The Maintenance of Lipid Asymmetry (Mla) pathway is a multicomponent system found in all gram-negative bacteria that contributes to virulence, vesicle blebbing and preservation of the outer membrane barrier function. The pathway consists of an OM lipoprotein component (MlaA), found as part of a complex with either OmpC or OmpF7,8; a periplasmic GPL chaperone (MlaC) which shuttles GPL across the periplasm; and an IM ATP binding cassette (ABC) transporter complex (MlaFEDB). MlaFEDB consists of four proteins: MlaE an ABC permease protein; MlaD a membrane anchored MCE (mammalian cell entry) domain containing protein forming a homo-hexameric ring that faces the periplasm; MlaF, an ABC ATPase; and MlaB, a STAS (Sulfate Transporter and Anti-Sigma factor antagonist) domain protein proposed to have a regulatory function. Specifically, we report the structure of E. coli MlaC in complex with the MlaD hexamer, in two different stoichiometries (1:6 and 2:6, respectively), stabilised through the binding of cardiolipin.

Masked refinement and 3D classification, focusing on one MlaD hexamer, revealed two distinct species, one with a single MlaC bound to a MlaD32-183 hexamer, and another with two MlaC molecules bound, with final resolutions of 4.35 Å and 4.38 Å, respectively. In the MlaCD(2:6) structure, two MlaC molecules are bound on opposite sides of the MlaD32-183 hexamer, with overall 2-fold symmetry. Likewise, MlaCD(2:6) has a Cɑ RMSD of between 0.7 and 0.9 Å in the core fold across all pairwise protomer alignments, except for those positioned directly opposite in the hexamer, which have RMSDs as low as 0.3 Å in the core fold and 0.4 Å for the entire Cɑ trace. Further 2D and 3D classification of the data did not reveal any evidence for particles with additional copies of MlaC bound to the MlaD32-183 hexamer, or for any MlaCD(2:6) structures with the two MlaC monomers bound in any orientation other than directly opposite each other. We believe our complex structure adopts a more realistic native-like arrangement than that obtained by MacRae et al. who used a multidentate MlaC ligand which likely promoted a non-physiological binding arrangement with MlaC molecules bound at positions MlaD1 and MlaD3, rather than the MlaD1 and MlaD4 directly opposite orientation we observed. The MlaCD(2:6) structure is also consistent with the observed two-fold symmetry for the MlaFEB components. The interaction interface itself is made up of predominantly electrostatic interactions, with MlaD32-183 forming a largely electronegative surface, composed of residues from β5, β6, β8 and α1 together with the β6-β7 loop, whilst MlaC features a positively charged groove that complements the negatively charged β6-β7 loop of MlaD, composed of residues found within helices α3, α4, α6, the β4-α6 loop and β2-β3 loop. However, binding to MlaD, between the β6-β7 loop and the main body could pull the GPL binding cavity open allowing GPLs to enter.

>MQTKKNEIWVGIFLLAALLAALFVCLKAANVTSIRTEPTYTLYATFDNIGGLKARSPVSIGGVVVGRVADITLDPKTYLPRVTLEIEQRYNHIPDTSSLSIRTSGLLGEQYLALNVGFEDPELGTAILKDGDTIQDTKSAMVLEDLIGQFLYGSKGDDNKNSGDAPAAAPGNNETTEPVGTTK[6x];>MFKRLMMVALLVIAPLSAATAADQTNPYKLMDEAAQKTFDRLKNEQPQIRANPDYLRTIVDQELLPYVQVKYAGALVLGQYYKSATPAQREAYFAAFREYLKQAYGQALAMYHGQTYQIAPEQPLGDKTIVPIRVTIIDPNGRPPVRLDFQWRKNSQTGNWQAYDMIAEGVSMITTKQNEWGTLLRTKGIDGLTAQLKSISQQKITLEEKK[2x]> ASMQKLINSVQ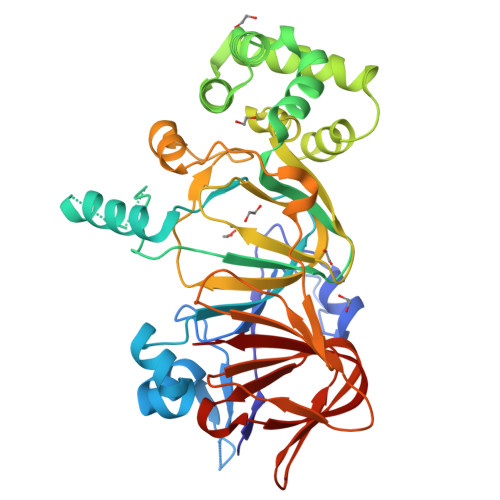NYAWGSKTALTELYGIANPQQQPMAELWMGAHPKSSSRITTANGETVSLRDAIEKNKTAMLGEAVANRFGELPFLFKVLCAAQPLSIQVHPNKRNSEIGFAKENAAGIPMDAAERNYKDPNHKPELVFALTPFLAMNAFREFSDIVSLLQPVAGAHSAIAHFLQVPNAERLSQLFASLLNMQGEEKSRALAVLKAALNSQQGEPWQTIRVISEYYPDDSGLFSPLLLNVVKLNPGEAMFLFAETPHAYLQGVALEVMANSDNVLAAGLTPKYIDIPELVANVKFEPKPAGELLTAPVKSGAELDFPIPVDDFAFSLHDLALQETSIGQHSAAILFCVEGEAVLRKDEQRLVLKPGESAFIGADESPVNASGTGRLARVYNKL> GEDTALVRPVKTATVSSQSVILKDFSGMVEAVEYVKLAFRVSGQIINLPVVEGQRVKKGQLIAAIDPRDISLQYAADKAAYETAAAQVERNKRLLGRQAISLQEYEISVANYQKAKSAYELSTNNMRDTKLLAPFDGSIETRLVENYQRVNSGEGIVRLVNTRKLRIKFTVPDDYLYLLRAKDATFKVEFDTYKGTVFNARLEEYLDISTDGTGIPVTIIIDDAAFDRTIYDVKPGFTCNIRLASDIAPFIEEKLMNVPLSAVFGDSENKNTYVWIVKDNKVNRREVTVYSPTGEANLLISKGLKPGETVVTAGVYQLVEGQ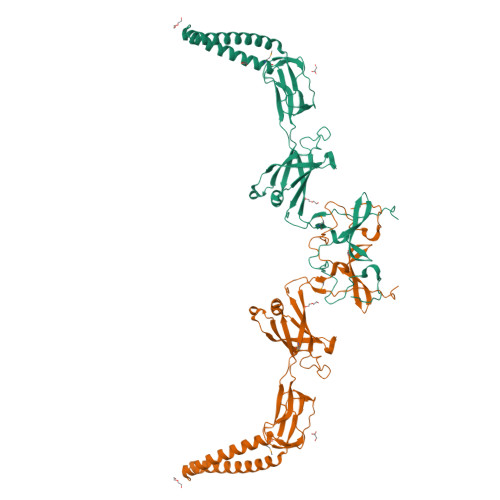RIKEVK> MKINDDIKELILEYMSRYFKFENDFYKLPGIKFTDANWQKFKNGGTDIEKMGAARVNAMLDCLFDDFELAMIGKAQTNYYNDNSLKMNMPFYTYYDMFKKQQLL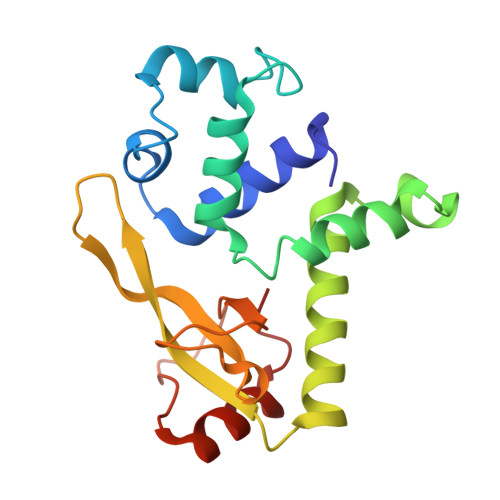KWLKNNRDDVIGGTGRMYTASGNYIANAYLEVALESSSLGSGSYMLQMRFKDYSKGQEPIPSGRQNRLEWIENNLENIR> MTKVVEISPTTRLEGHSKLTLKVNDQGIVERGDWLSITPVRGIEKLAIGKTMEQVPKIASRVCGICPIAHTLASTEAMEASIGCEIPTDAKLLRIILHAANRIHSHALHNILILPDFYIPGTEKKFNLFANEQPARSVMARIVRIREIAQTIAAIAGGEAIHPSNPRIGGMYHNVSPRAKQKMADLAKECLVLVHEQMEFMLDVIRNMQNREFVEVGGKQIPLPKKLGYHNQGVMATAPMYGSSSLDDNPTWDFTRWKETRPWDWYMGEVTIDLEDPSYPIGGTTKVGTKANPQMESCTGVPTYDGQPVEVGPRARLATFKNFDEKGTFAQHIARQMEYPDCCYTILNCLDNLNTSGKVLADHIPQGDGSMGWAANEAPRGSNIHLARVKDGKVRWYDMLVPTTWNFPTCSRALTGAPWQIA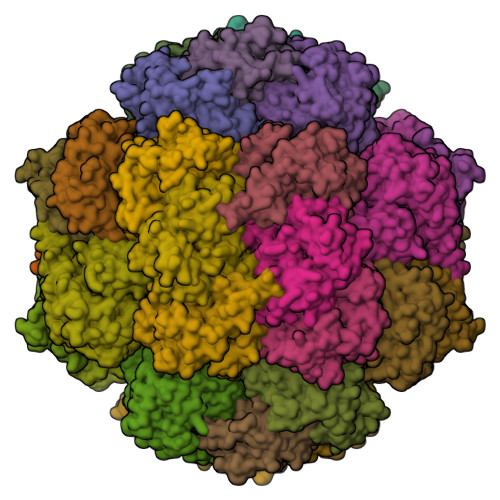EMVVRAYDPCVSCATH;> MIEDPYLGKYVTCVSARSTDKEILKKAQDGGIATALMVYALEEGFIDGTIVAGEGDKPWQPKPVVAMTREDILKARGTRYNISPQISWLKEATRSFGLDKVGVTGVCCQMQAVRKAQLYPINMRDVPGKVAFTVGLFCMENFSYKSLQSIVEDHANQSLGSVKKMEITKGKFWVYTERGNVATVPLKATHKYEQPGCHVCLDYVSNLADISTGSVGSPDGWSTVFIRTKVGNEIWSKAVADGMFETKPIEEVKPGLDLLRKLAKQKIDKNQKTVEERKTFGINKGLRNPYA;> TNKIKIGHVHMSGCTGCLVSLADNNLGLIKILDDYADLVYCLTLADVRHIPEMDVALVEGSVCLQDHESVEDIKETRKKSKIVVALGSCACYGNITRFSRGGQHNQPQHESYLPIGDLIDVDVYIPGCPPSPELIRNVAVMAYLLLEGNEEQKELAGKYLKPLMDLAKRGTSGCFCDLMYDVINQGLCMGCGTCAASCPVHAITLEFGKPQGERDLCIKCGSCYGACPRSFFNLDVISEFENISEIIAKALKD>GNSN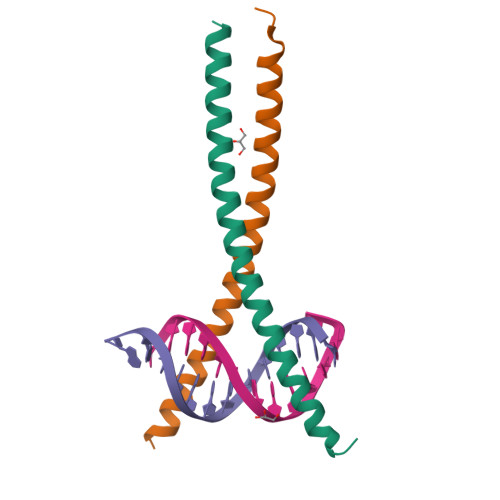EYRVRRERNNIAVRKSRDKAKQRNVETQQKVLELTSDNDRLRKRVEQLSRELDTLRG[2x]>MTKFSGNELRAELYRRAFLSYSVAPGALGMFGRSLLAKGARAEALANGTVMSGSHWGVFTATVENGRATAFTPWEKDPHPSPMLAGVLDSIYSPTRIKYPMVRREFLEKGVNADRSTRGNGDFVRVSWDQALDLVAAEVKRVEETYGPEGVFGGSYGWKSPGRLHNCTTLLRRMLTLAGGYVNGAGDYSTGAAQVIMPHVVGTLEVYEQQTAWPVLAENTEVMVFWAADPIKTSQIGWVIPEHGAYPGLEALKAKGTKVIVIDPVRTKTVEFFGAEHITPKPQTDVAIMLGMAHTLVAEDLYDKDFIANYTSGFDKFLPYLDGETDSTPKTAEWAEGISGVPAETIKELARLFESKRTMLAAGWSMQRMHHGEQAHWMLVTLASMLGQIGLPGGGFGLSYHYSGGGTPSTSGPALAGITDGGAATKGPEWLAASGASVIPVARVVDMLENPGAEFDFNGTRSKFPDVKMAYWVGGNPFVHHQDRNRMVKAWEKLETFVVHDFQWTPTARHADIVLPATTSYERNDIETIGDYSNTGILAMKKIVEPLYEARSDYDIFAAVAERLGKGAEFTEGKDEMGWIKSFYDDAAKQGKAAGVQMPAFDAFWAEGIVEFPVTDGADFVRYASFREDPLLNPLGTPTG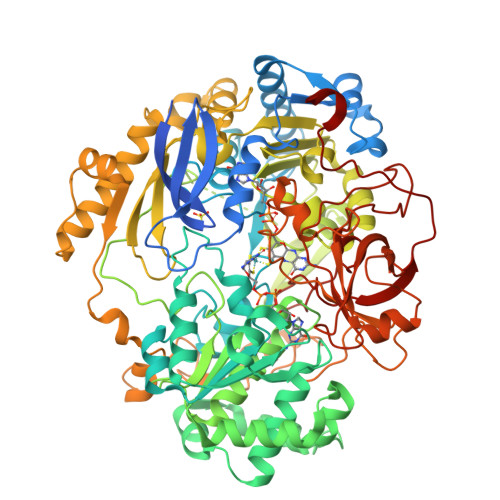LIEIYSKNIEKMGYDDCPAHPTWMEPLERLDGPGAKYPLHIAASHPFNRLHSQLNGTVLREGYAVQGHEPCLMHPDDAAARGIADGDVVRVHNDRGQILTGVKVTDAVMKGVIQIYEGGWYDPSDVTEPGTLDKYGDVNVLSADIGTSKLAQGNCGQTVLAEVEKYTGPAVTLTGFVAPKAAE[2x]>[4x]GIG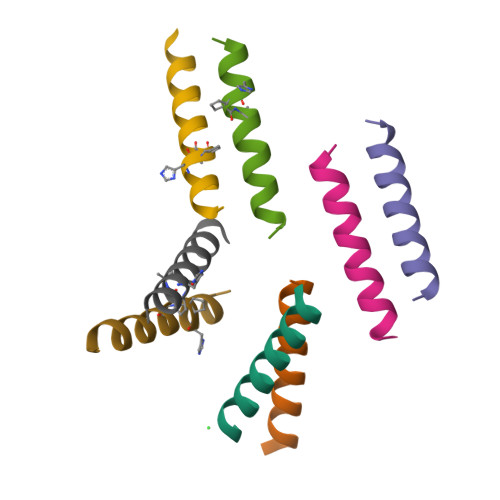KFLHAAKKFAKAFVAEIMNS;>[4x]GIGKFLHXAKKFAKAFVAEIMNS>GSPKNLINIDKPIKELPASIAIPKEKPLTGEQQKMYDEVLKHFSNPDLKVYTS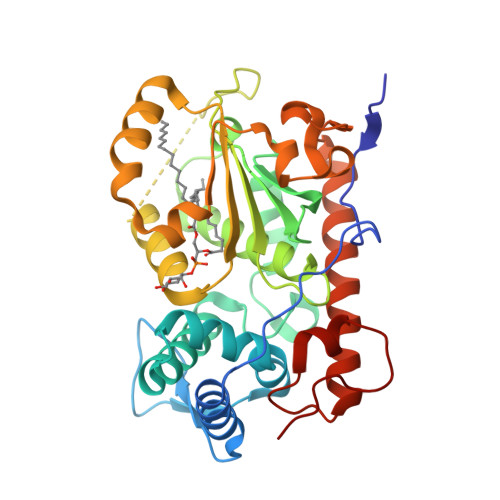EKNKSEDDLKPLEEEEKAWLTRECFLRYLRATKWVLKDCIDRITMTLAWRREFGISHLGEEHGDKITADLVAVENESGKQVILGYENDARPILYLKPGRQNTKTSHRQVQHLVFMLERVIDFMPAGQDSLALLIDFKDYPDVPKVPGNSKIPPIGVGKEVLHILQTHYPERLGKALLTNIPWLAWTFLKLIHPFIDPLTREKLVFDEPFVKYVPKNELDSLYGGDLKFKYNHDVYWPALVETAREKRDHYFKRFQSFGGIVGLSEVDLRGTHEKLLYPVK[2x]>[2x]SEFMYFAGAKTGIYRAQTALISFIKQEIIQKISHQSWVIDLGIGKGQDLGRYLDAGVRHLVGIDKDQTALAELVYRKFSHATTRQHKHATNIYVLHQDLAEPAKEISEKVHQIYGFPKEGASSIVSNLFI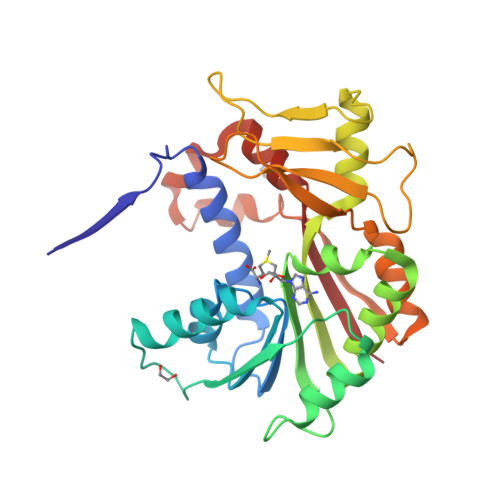HYLMKNTQQVENLAVLCHKLLQPGGMVWFTTMLGEQVLELLHENRIELNEVWEARENEVVKFAIKRLFKEDILQETGQEIGVLLPFSNGDFYNEYLVNTAFLIKIFKHHGFSLVQKQSFKDWIPEFQNFSKSLYKILTEADKTWTSLFGFICLRKN> MSSQAFTSVHPNAATSDVNVTIDTFVAKLKRRQVQGSYAIALETLQLLMRFISAARWNHVNDLIEQIRDLGNSLEKAHPTAFSCGNVIRRILAVLRDEVEEDTMSTTVTSTSVAEPLISSMFNLLQKPEQPHQNRKNSSGSSSMKTKTDYRQVAIQGIKDLIDEIKNIDEGIQQIAIDLIHDHEILLTPTPDSKTVLKFLITARERSNRTFTVLVTEGFPNNTKNAHEFAKKLAQHNIETL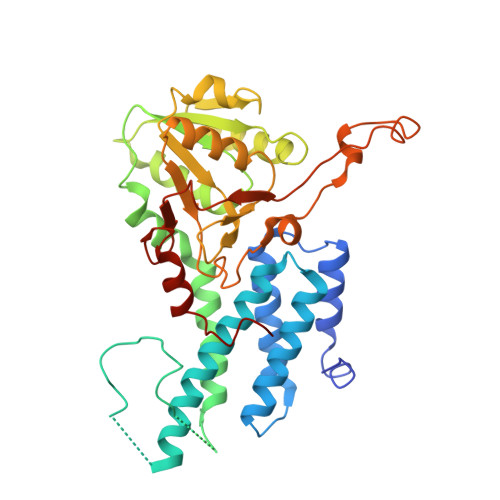VVPDSAVFALMSRVGKVIIGTKAVFVNGGTISSNSGVSSVCECAREFRTPVFAVAGLYKLSPLYPFDVEKFVEFGGSQRILPRMDPRKRLDTVNQITDYVPPENIDIYITNVGGFNPSFIYRIAWDNYKQIDVHLDKNKA N-{4-[{[(6S)-2-amino-4-oxo-3,4,5,6,7,8-hexahydropteridin-6-yl]methyl}(formyl)amino]benzoyl}-L-glutamic acid | 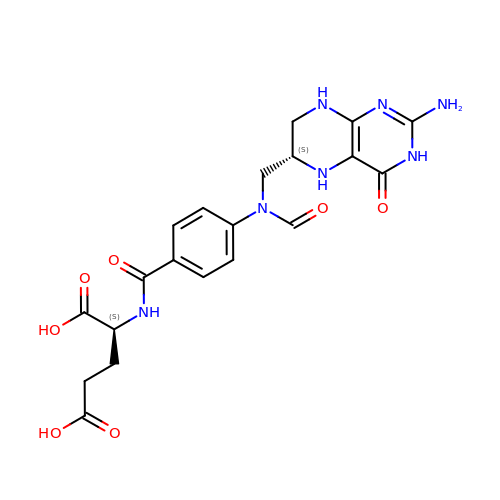C20 H23 N7 O7 | AUFGTPPARQZWDO-AAEUAGOBSA-N2-nonyl-4,6-bis(oxidanyl)benzoic 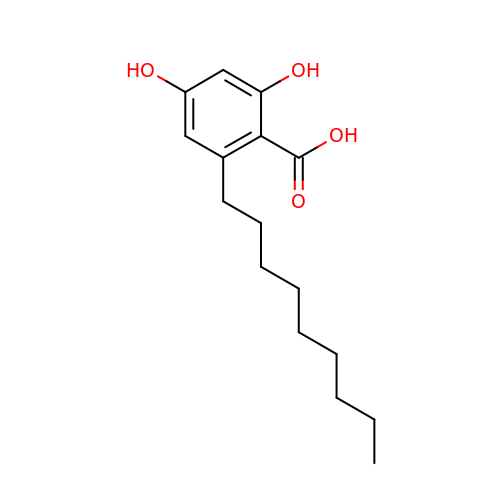acid | C16 H24 O4 | PTAHKOJJUSGQFK-UHFFFAOYSA-N> GSTSPVAQWEFHPGHFWMRGKR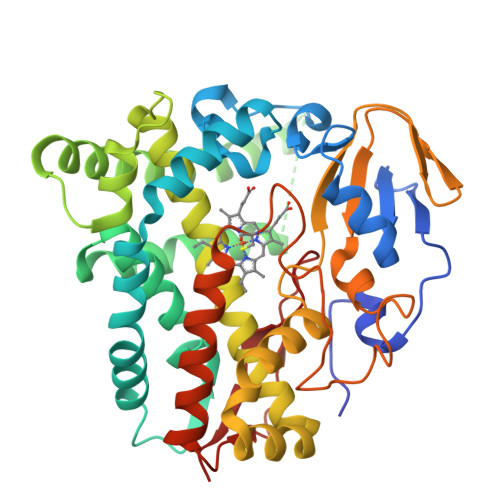PDKIVDYDEELQLWNVYGYPESAAILSNPKVFSSDTMRLDPIKLDEAIVEGDFAHTDPPKHRRLRGLVDHAFTPSLVAKMESRVHGIIHELLDGVEGKSQFDLVAEFAAPLPLIMISDLLGVPESDRALFRQWMDKMLDGSEKFESPETVLEQEEELHKELELLWEMRDYWHERAAESRKRPREDLISQLVHAEVDGQKLNDSQISNIANRLLVNGHLTTAMLIANTMLCLDAFSDQDARVRADRSLVPALLEESMRYMSPICGVGRATNSEVEVAGTVIPKDQLLLVWTGAANRDERQFEKPDVFDAGRSPNAHLGFGRGIHFCLGRQLARMESKAAVEILLDRLPTLRADPANPPTFLQVVDASGVATLPVVTQ> ECKEALAKSEMNVNMKYQLPNFTAETPIQNVILHEHHIFLGATNYIYVLNEEDLQKVAEYKTGPVLEHPDCFPCQDCSSKANLSGGVWKDNINMALVVDTYYDD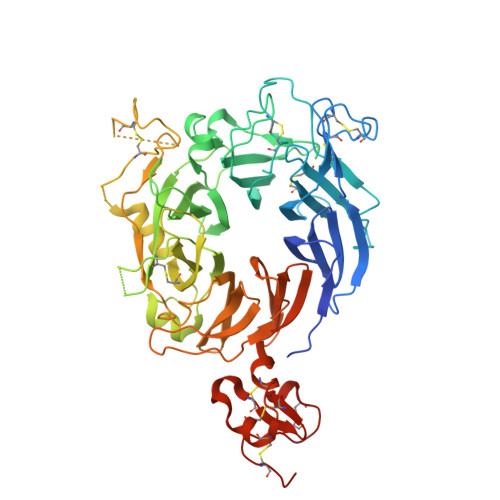QLISCGSVNRGTCQRHVFPHNHTADIQSEVHCIFSPQIEEPSQCPDCVVSALGAKVLSSVKDRFINFFVGNTINSSYFPDHPLHSISVRRLKETKDGFMFLTDQSYIDVLPEFRDSYPIKYVHAFESNNFIYFLTVQRETLDAQTFHTRIIRFCSINSGLHSYMEMPLECILTELVPRGSTKKEVFNILQAAYVSKPGAQLARQIGASLNDDILFGVFAQSKPDSAEPMDRSAMCAFPIKYVNDFFNKIVNKNNVRCLQHFYGPNHEHCFNRTLLRNSSGCEARRDEYRTEFTTALQRVDLFMGQFSEVLLTSISTFIKGDLTIANLGTSEGRFMQVVVSRSGPSTPHVNFLLDSHPVSPEVIVEHTLNQNGYTLVITGKKITKIPLNGLGCRHFQSCSQCLSAPPFVQCGWCHDKCVRSEECLSGTWTQQICLPAIYKHHHHHHHH6-O-phosphono-D-tagatose | C6 H13 O9 P | 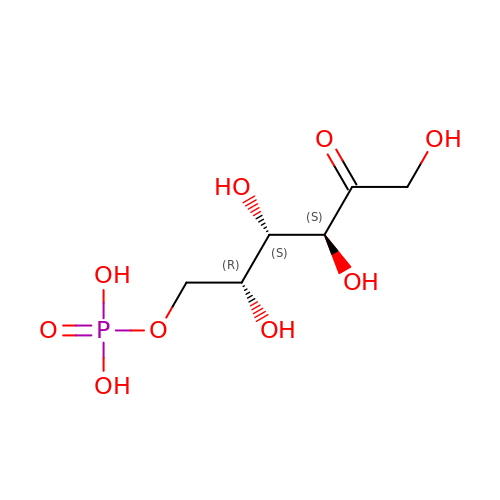GSXOAOHZAIYLCY-PBXRRBTRSA-N>[4x]GSHMGVGSVAALLTVVFYIAAVMATNLYGATFPEWFGDLSKSLYTLFQVMTLESWSMGIVRPVMNVHP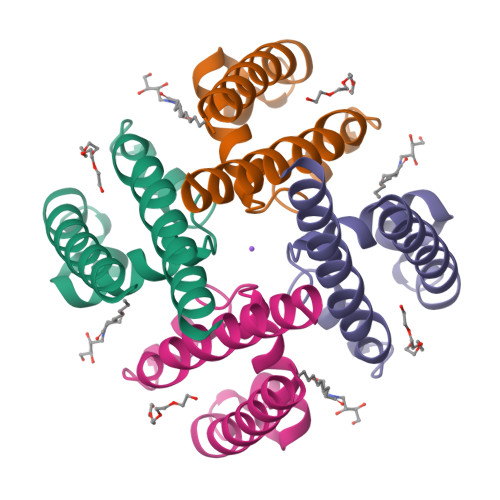NAWVFFIPFIMLTTFTVLNLFIGIIVDAMAITKEQEEEAKTGHHQEPISQTLLHLGDRLDRIEKQLAQNNELLQRQQPQKK>[2x]MKHHHHHHSAGLEVLFQGPGTGSEFMMFGKKKNNGGSSTARYSAGNKYNTLSNNYALSAQQLLNASKIDDIDSMMGFERYVPPQYNGRFDAKDIDQIPGRVGWLTNMHATLVSQETLSSGSNGGGNSNDGERVTTNQGISGVDFYFLDEEGGSFKSTVVYDPYFFIACNDESRVNDVEELVKKYLESCLKSLQIIRKEDLTMDNHLLGLQKTLIKLSFVNSNQLFEARKLLRPILQDNANNNVQRNIYNVAANGSEKVDAKHLIEDIREYDVPYHVRVSIDKDIRVGKWYKVTQQGFIEDTRKIAFADPVVMAFAIATTKPPLKFPDSAVDQIMMISYMIDGEGFLITNREIISEDIEDFEYTPKPEYPGFFTIFNENDEVALLQRFFEHIRDVRPTVISTFNGDFFDWPFIHNRSKIHGLDMFDEIGFAPDAEGEYKSSYCSHMDCFRWVKRDSYLPQGSQGLKAVTQSKLGYNPIELDPELMTPYAFEKPQHLSEYSVSDAVATYYLYMKYVHPFIFSLCTIIPLNPDETLRKGTGTLCEMLLMVQA;>MSINLHSAPEYDPSYKLIQLTPELLDIIQDPVQNHQLRFKSLDKDKSEVVLCSHDKTWVLKQRKHSNTVLLMREFVPEQPITFDETLLFGLSKPYMDVVGFAKTESEFETRETHGELNLNSVPIYNGELDFSDKIMKRSSTKVIGTLEELLENSPCSALEGISKWHKIGGSVKDGVLCILSQDFLFKALHVLLMSAMAESLDLQHLNVEDTHHAVGKDIEDEFNPYTREIIETVLNKFAVQEQEAENNTWRLRIPFIAQWYGIQALRKYVSGISMPIDEFLIKWKSLFPPFFPCDIDIDMLRGYHFKPTDKTVQYIAKSTLPMDPKERFKVLFRLQSQWDLEDIKPLIEELNSRGMKIDSFIMKYARRKRLGKKTVVTSR[2x];>MPSVDIDASQWQKLTQSREKQTTVITPLGMMMLEIQGELELPKDFASLARRDSPNEGRFSEQDGETLIRFGSLQIDGERATLFVGKKQRLLGKVTKLDVPMGIMHFNSKDNKVELVDVMKYKVIFKDRPLPIM[2x];>[2x]GAMGNQTVKIWVKYNEGFSNAVRKNVTWNNLWE

Ctf18-RFC belongs to the RFC family of AAA+ ATPase clamp loaders, which are involved in the loading and unloading of clamps onto dsDNA. Compared to other clamp loaders, Ctf18-RFC contains two additional subunits, Ctf8 and Dcc1, which bind to the C-terminus of Ctf18 to form the Ctf18-1-8 module. Mutations in Ctf18 that disrupt formation of this Ctf18-1-8 module result in similar but not identical phenotypes as entire deletions of Ctf18 (29,30), suggesting that this module is critical for at least some of the specialized functions of Ctf18-RFC. It has been shown that the Ctf18-1-8 module binds the N-terminal catalytic domain of Pol2 (30,31), the largest subunit of the leading strand Pol ϵ, and that this interaction increases the clamp loader activity of Ctf18-RFC.

Previously, we showed that the yeast Ctf18-1-8 module forms a relatively transient complex with a truncated construct of the Pol ϵ catalytic domain, Pol2(1–528), through the WH3 domain of Dcc1 (Dcc1WH3) and exonuclease domain of Pol2 (Pol2EXO). Although this minimal complex could be disrupted in vitro by a structure-guided triple mutation, Dcc1 K364A/R376A/R380A (henceforth Dcc1-3A), a new crystal form of this complex revealed that this interface is highly flexible. The crystal structures provide an extreme example of this. Here, Dcc1WH3 has slid by 16 Å along the negatively charged Pol2EXO surface and forms entirely different molecular interactions with it. Although this conformation is presumably influenced by crystal contacts, approximately the same interface is utilized in two different crystal forms, suggesting it is a readily accessible state in the conformational continuum. Thus, our data show that the complex uses flexible electrostatic interfaces with low specificity that are readily adaptable to maintain tight complex formation in different conformational states.>[2x]LAAALEGPYPVEEIRLPRAGGPLGLSIVGGSDHSSHPFGVQEPGVFISKVLPRGLAARSGLRVG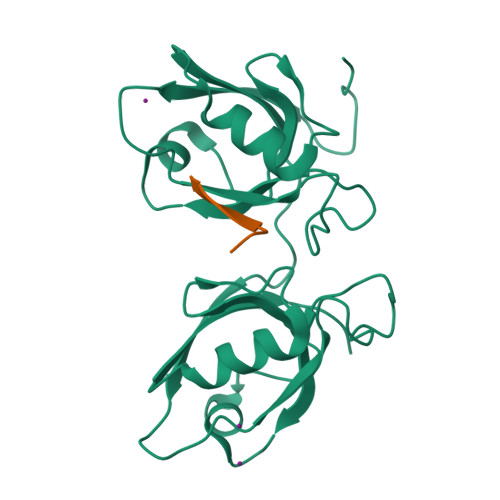DRILAVNGQDVRDATHQEAVSALLRPCLELSLLVRRDPAPPGLRELCIQKAPGERLGISIRGGARGHAGNPRDPTDEGIFISKVSPTGAAGRDGRLRVGLRLLEVNQQSLLGLTHGEAVQLLRSVGDTLTVLVCDGFEASTDAALEVS;>SWFQTDL[2x]>[4x]LGLSITGLGVQYPPYSLGPDAIDILSKRYHPESPAMKKVLAINRYTGIDQRSSIGNPDHPLVNKPNPPTVKELHEVFMSDGVPLAVEASRKAMAEARLVPAQITHMVSTTCTDSANPGYDHYVAKELGLSDRLEKVLLHGIGCSGGLAALRTAANLCLGHTARGKPARILVLALEVSTTMVRSELESIDALQETRIGIALFSDCASAVILSNGIG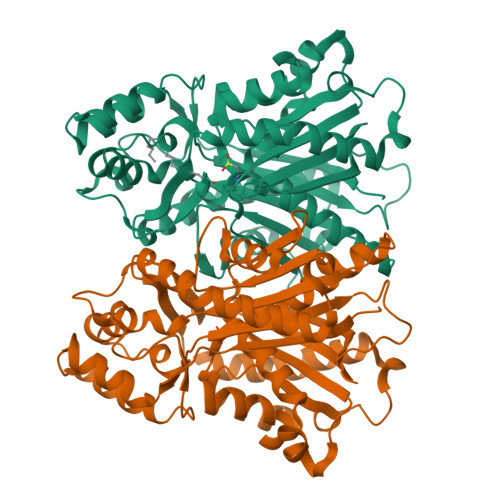EAPGKPAIYDLLGWENRVIPDSEHDLGFDVDPMGWKVVLSPRVPVLAKASLQPTYADLLSSLQDQLPSSYQKPADFDWAMHPGGATILSGAESAMGLTPEHMRASYDRYINHGNSSSATIFSVLNRLREKDMDALAPGGKVKEYVVGCAFGPGINVEMCMLKRR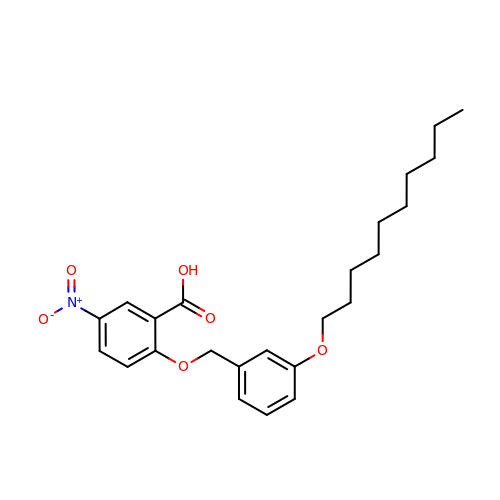2-{[3-(decyloxy)benzyl]oxy}-5-nitrobenzoic acid | C24 H31 N O6 | JVCSVSPXQNVWLW-UHFFFAOYSA-N>GUUAUGUGUGCCCGGCAUGGGUGCAGUCUAUAGGGUGAGAGUCCCGAACUGUGAAGGCAGAAGUAACAGUUAGCCUAACGCAAGGGUGUCCGUGGAAACAUGGAAUCUGAAGGAAGCGGACGGCAAACCUUCGGUCUGAGGAACACGAACUUCAUAUGAGGCUAGGUAUCAAUGGAUGAGUUUGCAUAACAAAACAAAGUCC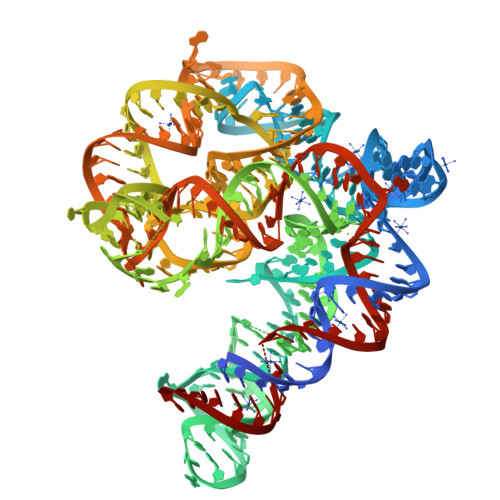UUUCUGCCAAAGUUGGUACAGAGUAAAUGAAGCAGAUUGAUGAAGGGAAAGACUGCAUUCUUACCCGGGGAUC[2x]>[4x]SQSRIFYLRNFNNWMKSVLIGEFLEKVRQKKKRDITVLDLGCGKGGDLLKWKKGRINKLVCTDIADVSVKQCQQRYEDMKNRRDSEYIFSAEFITADSSKELLIDKFRDPQMCFDICSCQFVCHYSFESYEQ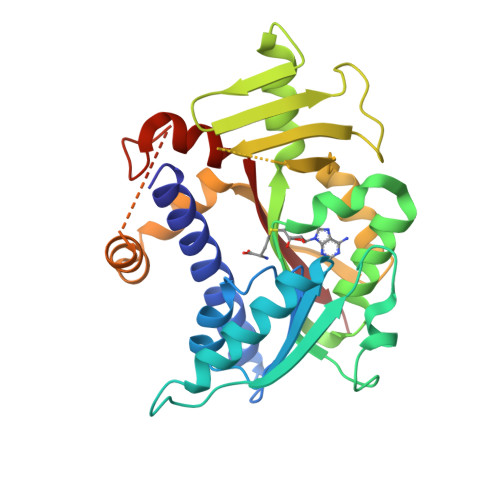ADMMLRNACERLSPGGYFIGTTPNSFELIRRLEASETESFGNEIYTVKFQKKGDYPLFGCKYDFNLEGVVDVPEFLVYFPLLNEMAKKYNMKLVYKKTFLEFYEEKIKNNENKMLLKRMQALEPYPANESSKLVSEKVDDYEHAAKYMKNSQVRLPLGTLSKSEWEATSIYLVFAFEKQQ>MGSKFIQNAAEIAKKAMDSVDPSLSEKFTIVIRFLTDNPDAASALKGKERSIVGTEEYIIASATNFKKGRDPRTPLPPSTIPDEMVSVILNKYFEVPSEELEKAEEWHRLSMGAENIVGDLLERYIAEVIEPHGWIWCSGSMVRAVDFIYCDSENVWQSLQVKNRDNTENSSSAAIRHGTPIKKWFRTFSKKRGDNWDKFPSLEGKENLSEKGFKLYVEKYLS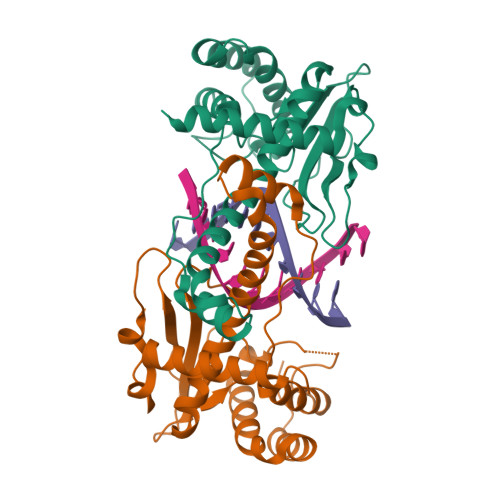ALRAIKALEHHHHHH[2x]>TKIP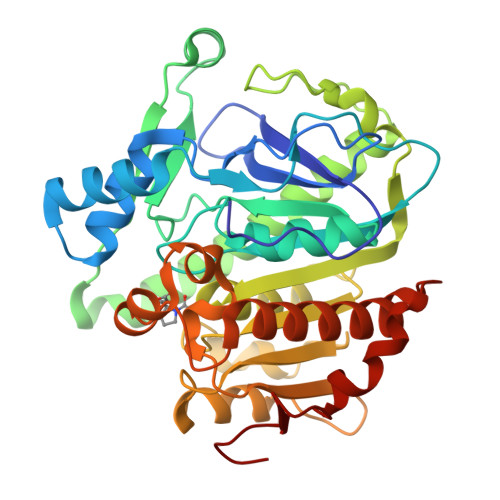RGNGPYSVGCTDLMFDHTNKGTFLRLYYPSQDNDRLDTLWIPNKEYFWGLSKFLGTHWLMGNILRLLFGSMTTPANWNSPLRPGEKYPLVVFSHGLGAFRTLYSAIGIDLASHGFIVAAVEHRDRSASATYYFKDQSAAEIGDKSWLYLRTLKQEEETHIRNEQVRQRAKECSQALSLILDIDHGKPVKNALDLKFDMEQLKDSIDREKIAVIGHSFGGATVIQTLSEDQRFRCGIALDAWMFPLGDEVYSRIPQPLFFINSEYFQYPANIIKMKKCYSPDKERKMITIRGSVHQNFADFTFATGKIIGHMLKLKGDIDSNVAIDLSNKASLAFLQKHLGLHKDFDQWDCLIEGDDENLIPGTNINT[2x]>[2x]HHHHHHHHHHMAVKKIAIFGATGQTGLTTLAQAVQAGYEVTVLVRDSSRLPSEGPRPA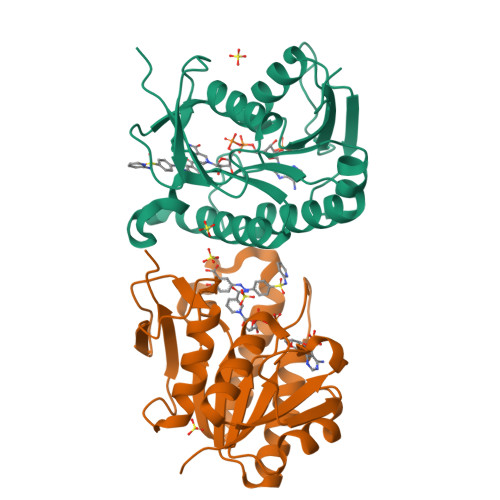HVVVGDVLQAADVDKTVAGQDAVIVLLGTRNDLSPTTVMSEGARNIVAAMKAHGVDKVVACTSAFLLWDPTKVPPRLQAVTDDHIRMHKVLRESGLKYVAVMPPHIGDQPLTGAYTVTLDGRGPSRVISKHDLGHFMLRCLTTDEYDGHSTYPSHQYQ> EDVEIKPRGYQLRLVDHLTKSNGIVYLPTGSGKTFVAILVLKRFSQDFDKPIESGGKRALFMCNTVELARQQAMAVRRCTNFKVGFYVGEQGVDDWTRGMWSDEIKKNQVLVGTAQVFLDMVTQTYVALSSLSVVIIDECHHGTGHHPFREFMRLFTIANQTKLPRVVGLTGVLIKGNEITNVATKLKELEITYRGNIITVSDTKEMENVMLYATKPTEVMVSFPHQEQVLTVTRLISAEIEKFYVSLDLMNIGVQPIRRSKSLQCLRDPSKKSFVKQLFNDFLYQMKEYGIYAASIAIISLIVEFDIKRRQAETLSVKLMHRTALTLCEKIRHLLVQKLQDMTYDDDDDNVNTEEVIMNFSTPKVQRFLMSLKVSFADKDPKDICCLVFVERRYTCKCIYGLLLNYIQSTPELRNVLTPQFMVGRNNISPDFESVLERKWQKSAIQQFRDGNANLMICSSVLEEGIDVQACNHVFILDPVKTFNMYVQSKGRARTTEAKFVLFTADKEREKTIQQIYQYRKAHNDIAEYLKDRVLEKTEPELYEIKGHFQDDIDPFTNENGAVLLPNNALAILHRYCQTIPTDAFGFVIPWFHVLQEDERDRIFGVSAKGKHVISINMPVNCMLRDTIYSDPMDNVKTAKISAAFKACKVLYSLGELNERFVPKTLKERVASIADVHFEHWNKYGDSVTATVNKADKSKDRTYKTECPLEFYDALPRVGEICYAYEIFLEPQFESCEYTEHMYLNLQTPRNYAILLRNKLPRLAEMPLFSNQGKLHVRVANAPLEVIIQNSEQLELLHQFHGMVFRDILKIWHPFFVLDRRSKENSYLVVPLILGAGEQKCFDWELMTNFRRLPQSHGSNVQQREQQPAPRPEDFEGKIVTQWYANYDKPMLVTKVHRELTPLSYMEKNQQDKTYYEFTMSKYGNRIGDVVHKDKFMIEVRDLTEQLTFYVHNRGKFNAKSKAKMKVILIPELCFNFNFPGDLWLKLIFLPSILNRMYFLLHAEALRKRFNTYLNLHLLPFNGTDYMPRPLEIDYSLKRNVDPLGNVIPTEDIEEPKSLLEPMPTKSIEASVANLEITEFENPWQKYMEPVDLSRNLLSTYPVELDYYYHFSVGNVCEMNEMDFEDKEYWAKNQFHMPTGNIYGNRTPAKTNANVPALMPSKPTVRGKVK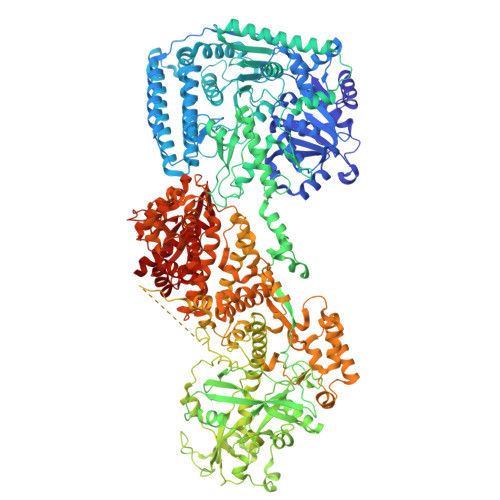PLLILQKTVSKEHITPAEQGEFLAAITASSAADVFDMERLEILGNSFLKLSATLYLASKYSDWNEGTLTEVKSKLVSNRNLLFCLIDADIPKTLNTIQFTPRYTWLPPGISLPHNVLALWRENPEFAKIIGPHNLRDLALGDEESLVKGNCSDINYNRFVEGCRANGQSFYAGADFSSEVNFCVGLVTIPNKVIADTLEALLGVIVKNYGLQHAFKMLEYFKICRADIDKPLTQLLNLELGGKKMRANVNTTEIDGFLINHYYLEKNLGYTFKDRRYLLQALTHPSYPTNRITGSYQELEFIGNAILDFLISAYIFENNTKMNPGALTDLRSALVNNTTLACICVRHRLHFFILAENAKLSEIISKFVNFQESQGHRVTNYVRILLEEADVQPTPLDLDDELDMTELPHANKCISQEAEKGVPPKGEFNMSTNVDVPKALGDVLEALIAAVYLDCRDLQRTWEVIFNLFEPELQEFTRKVPINHIRQLVEHKHAKPVFSSPIVEGETVMVSCQFTCMEKTIKVYGFGSNKDQAKLSAAKHALQQLSKCDA> MKTEWPELVGKSVEEAKKVILQDKPAAQIIVLPVGTIVTFEYRIDRVRLFVDRLDNIAQVPRV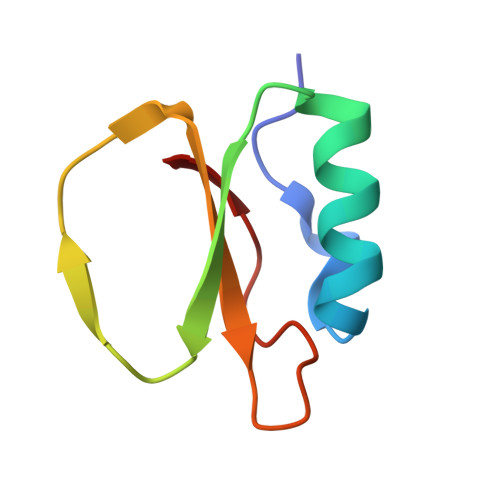G> MISNSSAESISAPPNDSTIPHLAIDPFSLDFFDDPYPDQQTLRDAGPVVYLDKWNVYGVARYAEVHAVLNDPTTFCSSRGVGLSDFKKEKPWRPPSLILEADPPAHTRPRAVLSKVLSPATMKTIRDGFAAAADAKVDELLQRGCIDAIADLAEAYPLSVFPDAMGLKQEGREHLLPYAGLVFNAFGPPNELRQTAIERSAPHQAYVNEQCQRPNLAPGGFGACIHAFTDTGEITPDEAPLLVRSLLSAGLDETVNGIGAAVYCLARFPGELQRLRSDPTLARNAF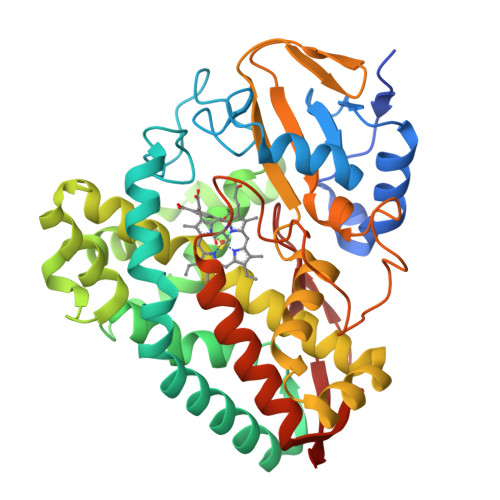EEAVRFESPVQTFFRTTTREVELGGAVIGEGEKVLMFLGSANRDPRRWSDPDLYDITRKTSGHVGFGSGVHMCVGQLVARLEGEVMLSALARKVAAIDIDGPVKRRFNNTLRGLESLPVKLTPA> SMGVAKLATIRTAGEITPIAGAEAIECCHVDGWTCVIKKGEFKQGDRGVYFEIDSFIKEDNDRYPMLSKQVIDYEGQRGTR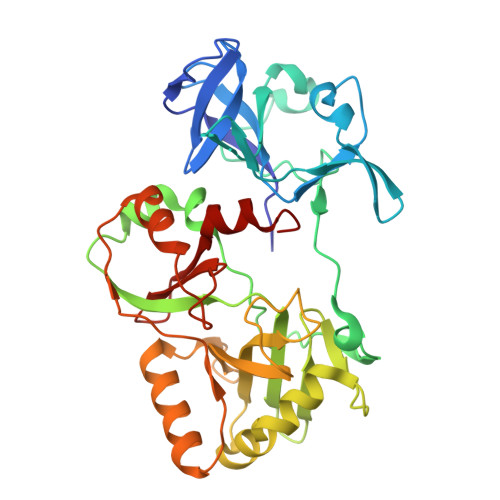LRTARLRGQLSQGLFLPMDRFPELASNQVGDDVTEILGITAWEPPISTNLSGEILGEFPTFISKTDQERVQNLIPQIEENKGQKFEVTVKLDGSSMTVYRKDDHIGVCGRNWELRETATNAQWHAARRNKMIEGLQFLNRNLALQGEIIGESIQGNLEKLKGQDFYLFDIYDIDKAQYLTPIERQSLVKQLNDNGFTVKHVPILDDLELNHTAEQILAMADGPSLNKNVKREGLVFKRLDGKFSFKAISNAYLEKHKDR(2R)-3-{[(R)-HYDROXY{[(1R,2R,3S,4R,5R,6S)-2,3,6-TRIHYDROXY-4,5-BIS(PHOSPHONOOXY)CYCLOHEXYL]OXY}PHOSPHORYL]OXY}PROPANE-1,2-DIYL DIBUTANOATE | C17 H33 O19 P3 | 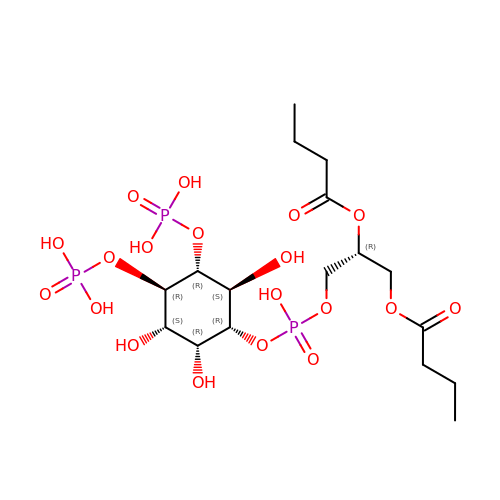DHAFWWKSHUBGAH-BXJBXBQISA-N6-{[(5-cyanopyrazin-2-yl)carbamoyl]amino}naphthalene-2-carboxylic 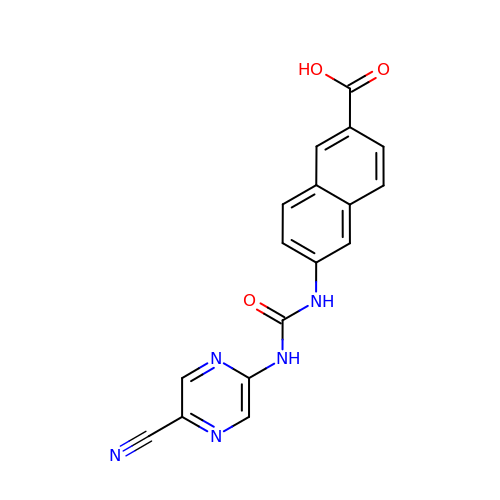acid | C17 H11 N5 O3 | CACMTVGXYAZZNY-UHFFFAOYSA-N>NLNLPEQSTRFQTIASIHSNNCSFEILNNDPGYIYGDSVDGECRIAVAHRELGNGLERTGDDRFLFIFYALDNNNFIIANRHDGFVLQFLIANGQGVIVSREYQPNIHQEFTIQSINSDTFRLHSRDTNTFATVCWAQFNSWTKIVSRVDNPGAPNANLKHRSLLTDINMPQLPSLTPLQPLPRLTELEDGGLSPAQAPRAIIGRTLIPCLFVNDPVLRLENRIKQSPYYVLEHRQYWHRIWTDIFTAGERREYREVTGINNNAQNDMNKMINITIGADGPNRLRFGNLSTPFRQQIIDNSNTLGSFANTNYGTRTDIVNVFNSEFHQVRYARFVKAYEYRLTRADGSQVGTPWVVLDRKEMDLRTYPHNMAITLENVKIDNADNSYDLSIWKTPLKLKDGKIIIENHENSKPYYN[2x]

The Cry48Aa/Tpp49Aa pair is produced by a number of L. sphaericus strains and is composed of Cry48Aa, a 135-kDa protein belonging to the 3-domain family of Crystal (Cry) proteins, and Tpp49Aa, a 53 kDa protein belonging to the family of Toxin_10 pesticidal proteins (Tpp). Mosquito toxicity bioassays have revealed that both components in combination are required for activity against Culex quinquefasciatus larvae. Within each Tpp49Aa1 monomer, two distinct domains exist: an N-terminal lectin-like head domain covering residues 49–214 and a C-terminal putative pore-forming domain (PFD) covering residues 215–464. The final model of Tpp49Aa1 revealed the presence of a homodimer forming an “X” structure with a large intermolecular interface, similar to that described for natural heterodimeric crystals of Tpp1Aa2/Tpp2Aa2.

Diffraction data were also collected following mixing with pH 3 buffer. In total, 466,741 diffraction patterns were collected from which 279,362 could be indexed in space group P212121, (a ~ 79.89; b ~ 82.84; c ~ 157.88 Å; α = β = γ = 90, highlighting an increase in unit-cell dimensions in comparison to the pH 7 dataset). Manual building and refinement from the ensembled diffraction data led to a model with Rwork/Rfree of 0.189/0.213 at 1.78 Å. Similar changes in the structure were seen following a decrease in pH from 7 to 3, although this is not physiologically relevant to pH values found in the target insect guts. Briefly, mixing at pH 3 results in a larger increase in overall binding energy at the eight crystal contacts (5.0 kcal mol−1) in comparison to mixing at pH 11 (1.8 kcal mol−1), suggesting that crystals may dissolve more readily at low pH.> MHHHHHHSSGRENLYFQGHMQVVAVRVWPASSYTRVTVESNRQLKYKQFALSNPERVVVDIEDVNLNSVLKGMAAQIRADD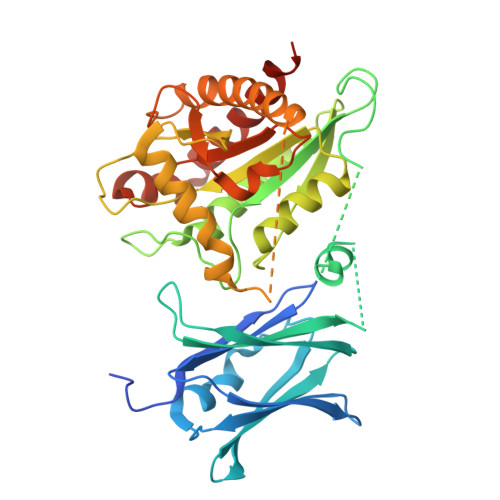PFIKSARVGQFDPQTVRMVFELKQNVKPQLFALAPVAGFKERLVMDLYPANAQDMQDPLLALLEDYNKGDLEKQVPPAQSGPQPGKAGRDRPIVIMLDPGHGGEDSGAVGKYKTREKDVVLQIARRLRSLIEKEGNMKVYMTRNEDIFIPLQVRVAKAQKQRADLFVSIHADAFTSRQPSGSSVFALSTKGATSTAAKYLAQTQNASDLIGGVSKSGDRYVDHTMFDMVQSLTIADSLKFGKAVLNKLGKINKLHKNQVEQAGFAVLKAPDIPSILVETAFISNVEEERKLKTATFQQEVAESILAGIKAYFADGATLARRG> AEAGITGTWYNQLGSTFIVTAGADGALTGTYESAVGNAESRYVLTGRYDSAPATDGSGTALGWTVAWKNNYRNAHSATTWSGQYVG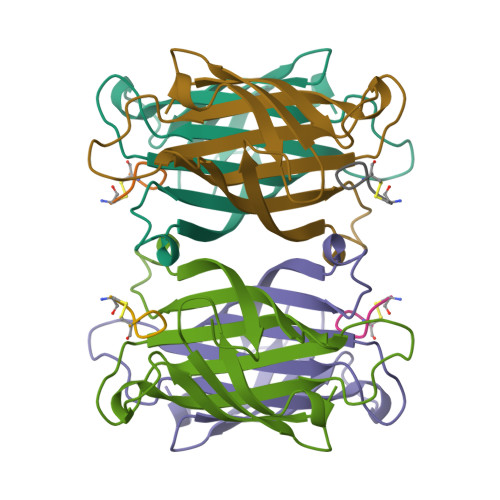GAEARINTQWLLTSGTTEANAWKSTLVGHDTFTKVKP> MTTLRAFTCDDLFRFNNINLDPLTETYGIPFYLQYLAHWPEYFIVAEAPGGELMGYIMGKAEGSV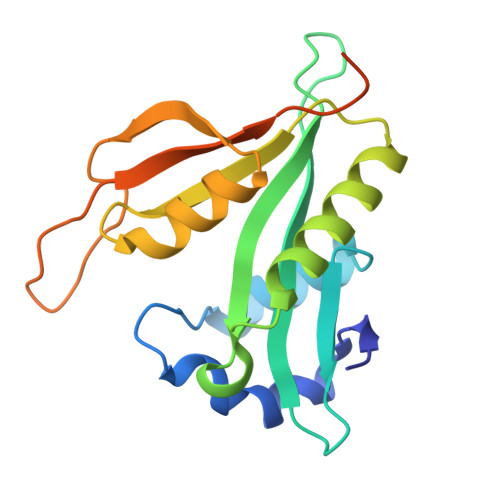AREEWHGHVTALSVAPEFRRLGLAAKLMELLEEISERKGGFFVDLFVRVSNQVAVNMYKQLGYSVYRTVIEYYSASNGEPDEDAYDMRKALSRDTEKKSIIPLPHPVRPEDIE> KISLLPPVNFTIKVTGLAQVLLQWKPNPDQEQRNVNLEYQVKINAPKEDDYETRITESKAVTILHKGFSASVRTILQNDHSLLASSWASAELHAPPGSPGTSIVNLTCTTNTTEDNYSRLRSYQVSLHCTWLVGTDAPEDTQYFLYYRYGSWTEECQEYSKDTLGRNIACWFPRTFILSKGRDWLAVLVNGSSKHSAIRPFDQLFALHAIDQINPPLNVTAEIEGTRLSIQWEKPVSAFPIHCFDYEVKIHNTRNGYLQIEKLMTNAFISIIDDLSKYDVQVRAAVSSMCREA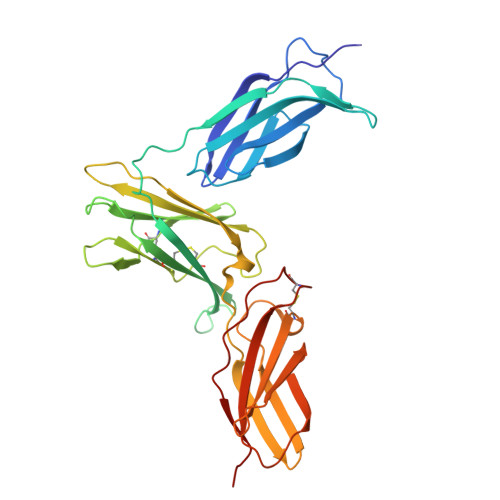GLWSEWSQPIYVGFSR> MNNLHRELAPVSDAAWEQIEEEATRTLKRFLAARRVVDVTDPQGAALSAVGTGHVAYLDGPCAGVSAVKRQVLPVVEFRVPFKLTRQAIDDVERGSQDSDWSPLKEAARKIAAAEDQTIFDGYMAAGIAGIRPQSSNTPLTLPATASDYPTVVAQALDQLRVAGVNGPYHLVLGEKAYTSITGGNEGGYPVFQHIRRLIDGEIVWAPAIEGGLLLTTRGGDFVMDIGQDISIGYLNHTGTDVELYLQESFTFSALTSEATVTLLPPEE;> MGCPFSQSVSQPVDERLTRAAIFLVVTINPGKAAEVAVRAHCSILSSLIRGVGFRI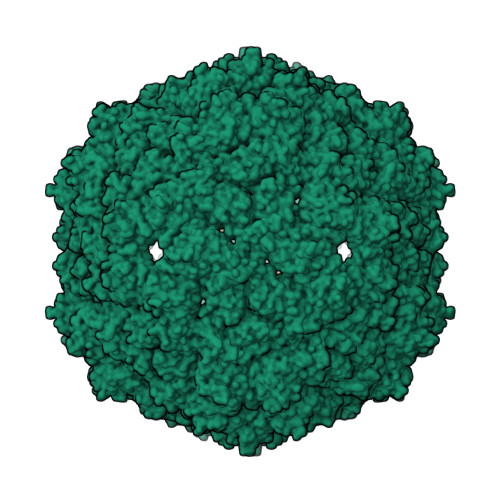SDGGLSCVMGVSEGGWERLFGDTKPEYLHVFREINGVHHAPSTPGDLLYHIRAARMDLCFELASRILSDLGNSVSVVDSVQGFRYFDDRDLLGFVDGTENPVAQAAVDATLIGDEDMVFAGGSYVIVQKYLHDLDKWNAIPVEQQEKIIGREKLSDIELRDADKPSYAHNVLTSIEEDGEDVDILRDNMPFGDPGKGEFGTYFIGYSRKPERIERMLENMFIGNPPGNYDRILDVSRAITGTLFFVPTTSFLDSIEPQSAPGQQGDDVINTLRSTAIKGDIMPGSLNIGSLKKEV(2~{S})-2-[[(2~{R})-2-[4-[(4-iodophenyl)carbonylamino]butanoylamino]-3-oxidanyl-3-oxidanylidene-propyl]carbamoylamino]pentanedioic acid 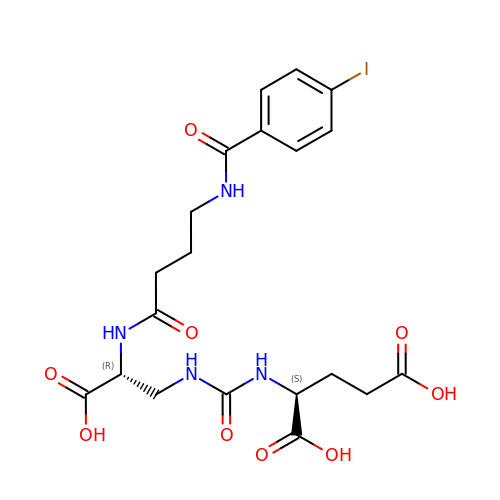| C20 H25 I N4 O9 | AOGSPOQTLUVJFT-UONOGXRCSA-N>[2x]MTKYFDYAASTPVAKGVLESMKPWQSDSFANPSAAHIEAEKALNAIKQAREIIADTLGAMPSEIVFTCGASESNNLAIKGLAFKRLEEKGHLITSSIEHKCVLNTCGFLESIGFDVTYLTPKASGLISAQQVEEAIRPNTFLITIHHVNNELGTVQPIEDIGNVAFEHDIPFHTDAAQSFCKLDIDVDDMNIDMLSLSGHKVYGPKGIGALYVRDARNSELVPLIHGGGQELGLRGGTSPTPLIVGLGVAVEHFPSEASAQQTEFEKIINEYSFSRNSGDNALSTTWNVTFENDDEVKRFTSERNWLISQGSASNAMSNTPSHVLTAIGLSEAEARRTYRISLPPYKV

Cysteine desulfurase, a pyridoxal phosphate (PLP)-dependent homodimer, strips sulfur from the l-cysteine substrate to generate l-alanine and a protein-bound persulfide intermediate on the active site cysteine residue. As a versatile sulfur donor, cysteine desulfurase activity is also essential to DNA phosphorothioate (PT) modification, in which the nonbridging oxygen atom in the DNA sugar-phosphate backbone is replaced by sulfur. In contrast to the typical dsDNA PT modification mediated by Dnd systems, Ssp systems confer single-stranded (ss), high-frequency DNA PT modification. SspA exhibits PLP-dependent cysteine desulfurase activity and is predicted to initiate the delivery of sulfur for ssDNA PT formation.

Here, we determined the crystal structure of the C314S mutant of SspA from V. cyclitrophicus FF75 in complex with its natural substrate, cysteine, at the resolution of 1.80 Å. In this structure, SspA forms a symmetric dimer, and its dimeric organization resembles that of other cysteine desulfurases, such as DndA and IscS. The SspA protein can be divided into two regions as follows: a larger N-terminal region (residues 1 to 254) possessing the PLP cofactor-binding site and a smaller C-terminal region (residues 255 to 348) bearing the Cys314 active site. The PLP cofactor is covalently attached to the side chain amino group of Lys201 in a deep surface pocket via the formation of an internal aldimine Schiff base. The imidazole ring of His99 forms π-π stacking with the pyridine ring of PLP to make multiple van der Waals interactions. In addition, the phosphate group of PLP forms hydrogen bonds with the side chains of Ser71, Ser198, and His200. In terms of the cysteine substrate, it is located in a positively charged surface pocket in SspA. The side chain guanidinium group of Arg340 and the side chain amide group of Asn150 make three hydrogen bonds with the carboxyl group of the cysteine substrate. The distance between Cys314 and the PLP cofactor is approximately 14.4 Å, and the distance between Cys314 and the cysteine substrate is 8.9 Å. In addition, although the distance between the catalytic Cys314 and the substrate cysteine is 8.9 Å, which is too far for direct interaction, our structural modeling and biochemical analysis revealed a conformational change in the active site region toward the cysteine substrate to move them close to each other to facilitate the nucleophilic attack.> VDQATLDKLEAGFKKLQEASDCKSLLKKHLTKDVFDSIKNKKTGMGATLLDVIQSGVENLDSGVGIYAPDAESYRTFGPLFDPIIDDYHGGFKLTDKHPPKQWGDINTLVGLDPAGQFIISTRVRCGRSLQGYPFNPCLTAEQYKEMEEKVSSTLSSMEDELKGTYYPLTGMSKATQQQLIDDHFLFKEGDRFLQTANACRYWPTGRGIFHNDAKTFLVWVNEEDHLRIISMQKGGD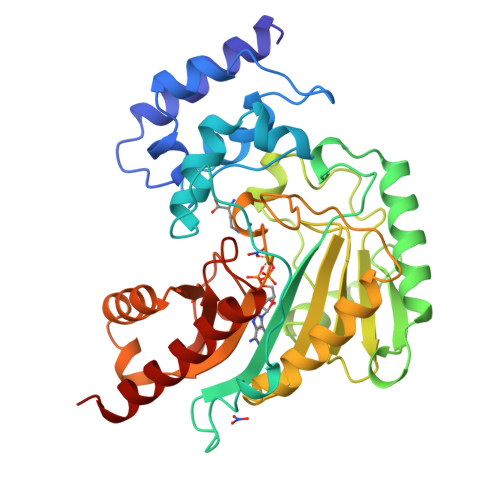LKTVYKRLVTAVDNIESKLPFSHDDRFGFLTFCPTNLGTTMRASVHIQLPKLAKDRKVLEDIASKFNLQVRGTRGEHTESEGGVYDISNKRRLGLTEYQAVREMQDGILEMIKMEKAAA>SNAMKIIDKLYEKVSKNGFVCIGLDSSIDYIPENMKAGKSVSEALFSYNKEIIDQTYDVCAIYKLQIAYYESYGIEGMIAYRDTLSYLREKDLLSIGDVKRSDIAASAKMYAKAHFEGDFETDFITLNPYMGMDSIEPYEEYIEKGDKGVFVLLRTSNPGAKDFEVLPVDGEEFFYKVGDKMRELNEKYIGKSGFGPIGLVVGATHSEEVEKIRKRYDKMFFLIPGFGAQKADSM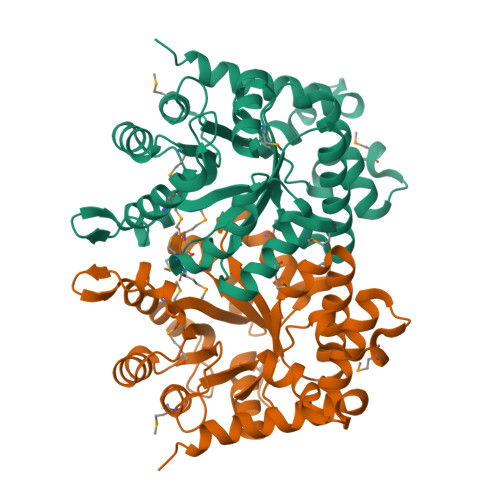NVYKLLEGLNGGVVNSSRAILKNWQNYEDGSEKVGYYARKKAIETYEEIKANEVL[2x]> MNQSSLLAEFGDPITRVENALQALREGRGVLLLDDEDR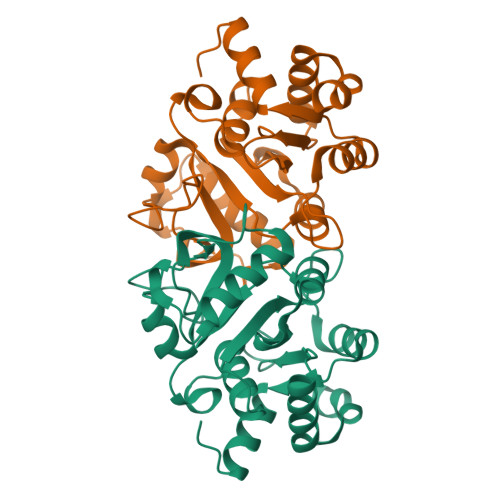ENEGDIIYAVESLTTAQMALMIRECSGIVCLCLTEAQADRLALPPMVVNNNSANQTAFTVSIEAKHGVTTGVSAQDRVTTIKTAANPQAKPEDLARPGHVFPLRARAGGVLARRGHTEGTVDLMQMAGLQPAGVLCELTNPDGSMAKTPEIIEFGKLHNMPVLTIEDMVQYRIQFDLKLA> MQQLNENKIIKLLRDNIPKLQLIYLFGSYSQGTQHRNSDIDIAVLAADTLDNIARWELAQKLASALDSDVDLVDLRSASTVLCQQVVTQGKQLWGTQQDDELFAVKTISMYQHLQAERQAIIDDVMANTAAKAHRGESL;>[3x]MNDIIINKIATIKRCIKRIQQVYGDGSQFKQDFTLQDSV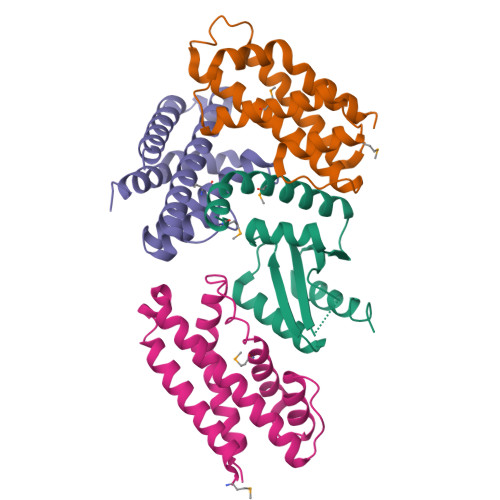ILNLQRCCEACIDIANHINRQQQLGIPQSSRDSFTLLAQNNLITQPLSDNLKKMVGLRNIAVHDYQELNLDIVVHVVQHHLEDFEQFIDVIKAEHHHHHH> RW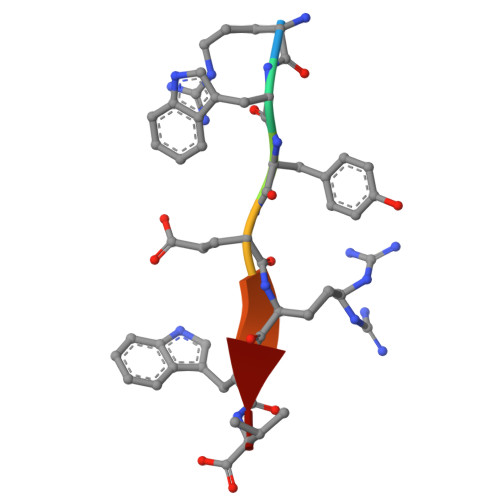YERWV> GPHMKS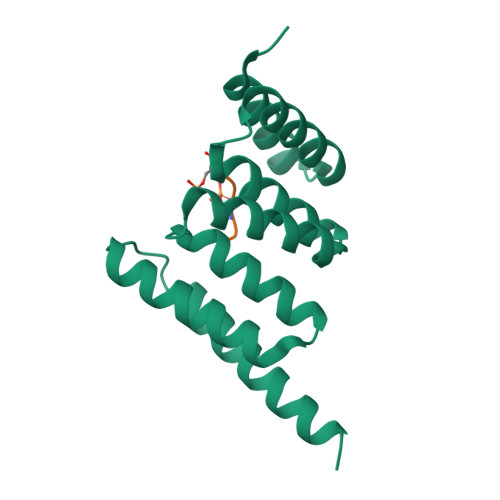PSAQELKEQGNRLFVGRKYPEAAACYGRAITRNPLVAVYYTNRALCYLKMQQPEQALADCRRALELDGQSVKAHFFLGQCQLEMESYDEAIANLQRAYSLAKEQRLNFGDDIPSALRIAKKKRWNSIEERR;> SPHNPISSVS>[4x]MSYYHHHHHHLESTSLYKKAGLENLYFQGMATPPKRSSPSFSASSEGTRIKKISIEGNI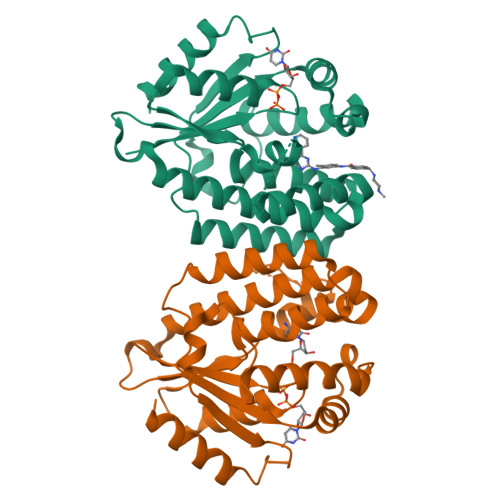AAGKSTFVNILKQLSEDWEVVPEPVARWSNVQSTQDEFEELTMSQKNGGNVLQMMYEKPERWSFTFQTYACLSRIRAQLASLNGKLKDAEKPVLFFERSVYSDRYIFASNLYESECMNETEWTIYQDWHDWMNNQFGQSLELDGIIYLQATPETCLHRIYLRGRNEEQGIPLEYLEKLHYKHESWLLHRTLKTNFDYLQEVPILTLDVNEDFKDKYESLVEKVKEFLSTL> DKSIEVGRX;> MGSSHHHHHHSQLEVLFQGPLGSGRPKKVPSAQTAYSVELARNLTWRRERKALLQEKKGLVNGNGTEMTSVQFPPPPNLAASAPRRSSLGFTLDLHRIQRDYIDLVPKHWHVISLSLSDGGHDLCITRLQAGQAPFVLRLPLERASSRDSSVDETDVFDFHTGRAELLEIIKEINRTCHDSRDMAAKGEREKWWAEREALDQRLKELLMNIEHVWLGGFRGVFSQHGRRPELLEKFRAMFEGVLDKHLP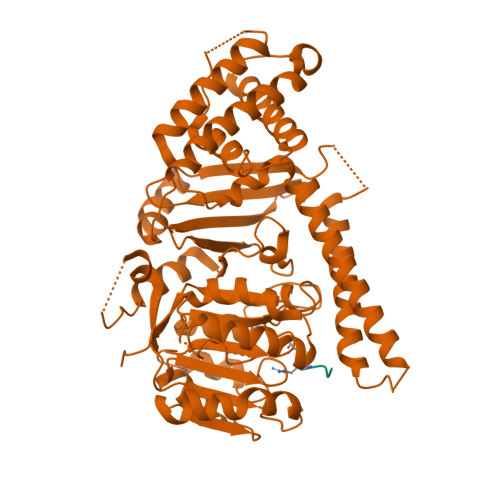SRRQVGRGKKGKGVAGQTKVVLDGNVLELFIGLGDATKSGADFDEELTDLLYFVVDILQFHGERNAYDEIDFDSMVVETMDALMAYHAEANAAPESDSHAHTILVLDKQLHVFPWESLPCLQGLAVSRIPSLACLRKLLLDRRRSSSQIQGEDSEEEDPRSAGHHAPLSGGTYILNPSSDLLSTQKTFESLFSTHLHSPNSWTRIISRPPTEPEFLSALTHSPILLYFGHGSGAQYIRSRNIRHLDHCRATVLLMGCSSAALTAKGEFEPSGPVWNYMLAGAPAVVGTLWDVTDRDIDRFAGGVLEGWGVLPEGCMGEKNGKKKAGRNGLSLVQAVAKARDRCRFRYVTAAAAVVYGIPVYVDVDGKSKD>[4x]GSALPILLDCDPGHDDAIAIVLALASPELDVKAITSSAGN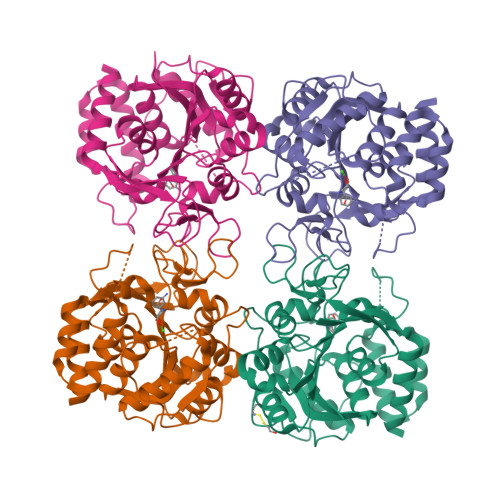QTPEKTLRNVLRMLTLLNRTDIPVAGGAVKPLMRELIIADNVHGESGLDGPALPEPTFAPQNCTAVELMAKTLRESAEPVTIVSTGPQTNVALLLNSHPELHSKIARIVIMGGAMGLGNWTPAAEFNIYVDPEAAEIVFQSGIPVVMAGLDVTHKAQIHVEDTERFRAIGNPVSTIVAELLDFFLEYHKDEKWGFVGAPLHDPCTIAWLLKPELFTSVERWVGVETQGKYTQGMTVVDYYYLTGNKPNATVMVDVDRQGFVDLLADRLKFYA> UGAGGUGNNGAGCGCG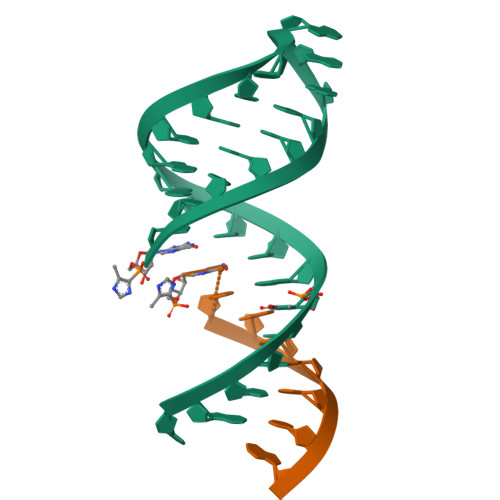AAAGCGCUC;> XCACCUCA> SNALRDLQKLNKDMVGWLTIIDTEIDYPILQSKDNDYYLHHNYKNEKARAGSIFKDYRNTNEFLDKNTIIYGHNMKDGSMFADLRKYLDKDFLVAHPTFSY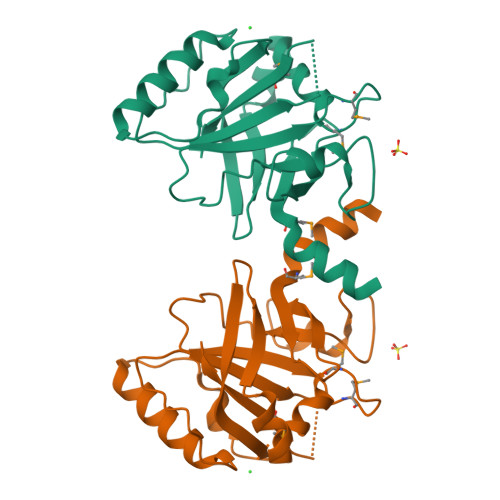ESGLTNYEVEIFAVYETTTDFYYIETEFPETTDFEDYLQKVKQQSVYTSNVKVSGKDRIITLSTCDTEKDYEKGRMVIQGKL>GPELDRASVQQLMEHFLAAYNEGDPRHLDHCLHPEYRHPNPAVERGIEGMRAAIRRWASTVEDLSLTLDDLVVEGDKAVARMTFSGRQVGPILGIPASGRRFSVGLIDIFLIEDGLFAQHWDEMDLLGLHRQLGALPD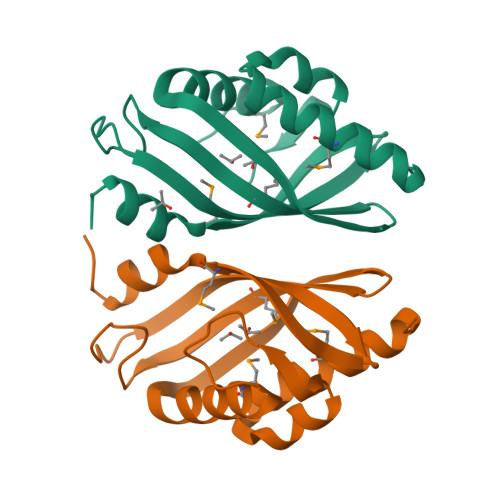[2x]> RCELKLIASPGSWRLYSARKIDERFKSYEQKIFQRDRYTCQFCGFQARLYQDIVNLDGDYTNNRLSNLVTACCFCAQCFFVESVGVGGYGGGTLIYLPELTQAELNSLCHVLFCAITNDTGYKSSAQNIYRSFKFRSQIVEEKFGEGTSDPA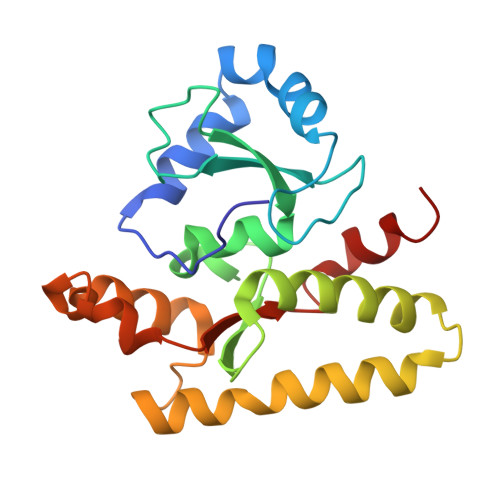IFGQLMIDSGVNSEEIREKLFKNIRLLPSRAKFRKQIEKWAAS>TTGHSYEKYNNWETIEAWTKQVTSENPDLISRTAIGTTFLGNNIYLLKVGKPGPNKPAIFMDCGFHAREWISHAFCQWFVREAVLTYGYESHMTEFLNKLDFYVLPVLNIDGYIYTWTKNRMWRKTRSTNAGTTCIGTDPNRNFDAGWCTTGASTDPCDETYCGSAAESEKETKALAD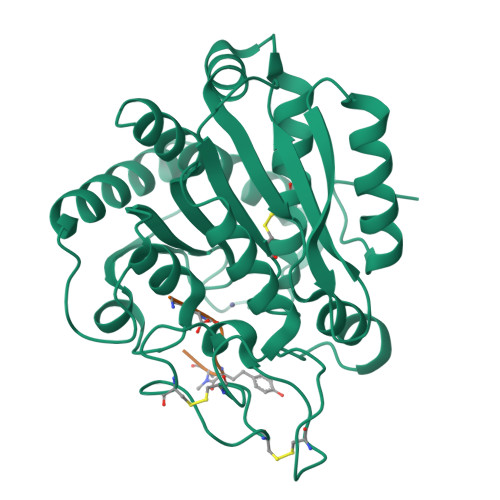FIRNNLSSIKAYLTIHSYSQMILYPYSYDYKLPENNAELNNLAKAAVKELATLYGTKYTYGPGATTIYPAAGGSDDWAYDQGIKYSFTFELRDKGRYGFILPESQIQATCEETMLAIKYVTNYVLGHL[3x];>[3x]KKVYAF> MVKKKTNNDKGKEVKENEGKLDIDSESSPHERENDKKKTEDDSLRATESEETNTHNANPNETVRADKFSQEESRPIEDSPHTDKNTAQESCQPSSAEDNVINTDITSLNEKTSTNDEQEKGLPLKISEGPFTISTLLDNVPSDLIYTCCEAYENHIFLGTTTGDLLHYFELERGNYMLVSQTKFDAESNSKIDKILLLPKVEGALILCDNELVLFILPEFAPRPNTTRLKGISDVVICNFSRSSKAYRIYAFHAEGVRLLKISADSLVLTKAFNFKLIDKACAHEETLMVSKLNSYELINLKSSQVIPLFRISETDEDLEPIITSFNEQSEFLVCSGGGSYDSGAMALVVNHHGDIIKGTIVLKNYPRNVIVEFPYIIAESAFQSVDIYSALPSEKSQLLQSITTSGSDLKISKSDNVFTNTNNSEEFKEKIFNKLRLEPLTHSDNKFRIERERAFVEESYEEKTSLIVYNNLGIHLLVPTPMVLRFTSCEESEIDNIEDQLKKLAKKDLTKFEHIEAKYLMSLLLFLMTLHYDHIEDEVMKKWCDFSDKVDIRILFYMFGWKVYSEIWCFHGLINIVERLKSLKLTNKCENILKMLLMMKNELKKKNKTGLLTNDFDDIMKTIDITLFKLRLEKKETITVDMFERESYDEIIREINLHDDKLPRIELLIEIYKEKGEYLKALNLLREAGDYISLVSFIEENLKKLPEDYIKERIADDLLLTLKQGDENTEECAIKKVLKILDMACINKNDFLNKIPAEETSLKVSFIEQLGVQNSNDSKFLFNYYLAKLREIINQSNIWSILGDFIKEYKDDFAYDKTDITNFIHIKLKHSLQCENFSKYYEKCENLKSENEKDDEFINFTFDEISKIDKEHILTLLFFPNELTNWVSSEELLKIYLSFNDFRSVEKYIGKQNLVAVMKQYLDISSLNYSVELVTNLLQRNFELLDDTDIQLKILETIPSVFPVQTISELLLKVLIKYQEKKEESNLRKCLL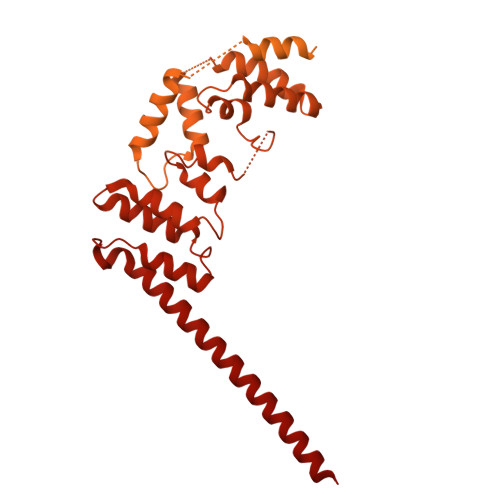KNQISISDELSRNFDSQG(methylsulfanyl)benzene | C7 H8 S | 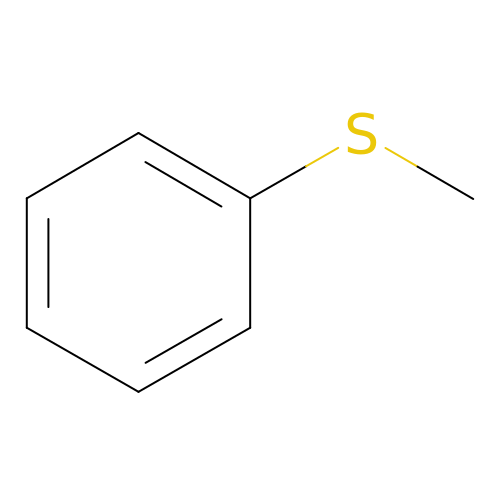HNKJADCVZUBCPG-UHFFFAOYSA-N>[2x]MNLVLMGLPGAGKGTQGERIVEKYGIPHISTGDMFRAAMKEETPLGLEAKSYIDKGELVPDEVTIGIVKERLGKDDCERGFLLDGFPRTVAQAEALEEILEEMGKPIDYVINIQV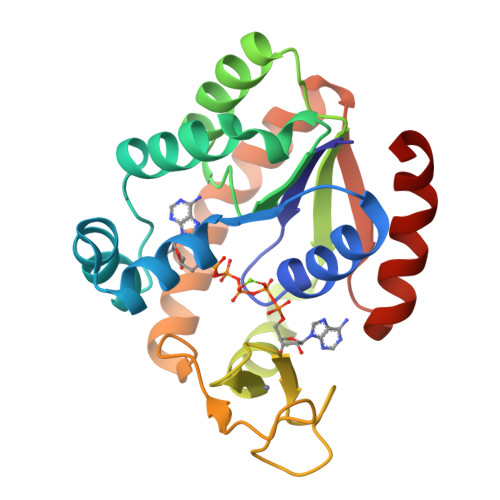DKDVLMERLTGRRICSVCGTTYHLVFNPPKTPGICDKDGGELYQRADDNEETVTKRLEVNMKQTAPLLDFYDEKGYLVNVNGQQDIQDVYADLKVLLGGLK> SMEQLKHCNGILKELLSKKHAAYAWPFYKPVDASALGLHDYHDIIKH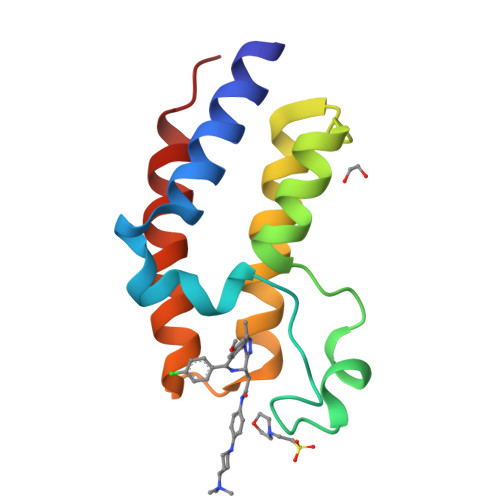PMDLSTVKRKMENRDYRDAQEFAADVRLMFSNCYKYNPPDHDVVAMARKLQDVFEFRYAKMPD> AINRLQLVATLVEREVMRYTPAGVPIVNCLLSYSGQAMEAQTARQVEFSIEA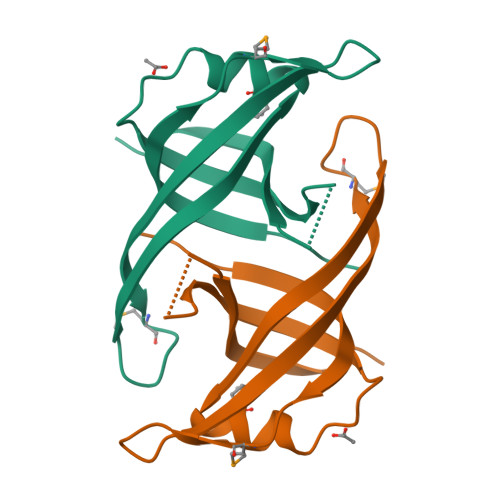LGAGKMASVLDRIAPGTVLDCVGFLARKHRSSKALVFHISGLEHHHHHH> MAPAVAGGGRVRSNEPVAAAAAAPAASGKPCVCGFQVCACTGSAAVASAASSLDMDIVAMGQIGAVNDESWVGVELGEDGETDESGAAVDDRPVFRTEKIKGVLLHPYRVLIFVRLIAFTLFVIWRISHKNPDAMWLWVTSICGEFWFGFSWLLDQLPKLNPINRVPDLAVLRQRFDRPDGTSTLPGLDIFVTTADPIKEPILSTANSVLSILAADYPVDRNTCYVSDDSGMLLTYEALAESSKFATLWVPFCRKHGIEPRGPESYFELKSHPYMGRAQDEFVNDRRRVRKEYDEFKARINSLEHDIKQRNDGYNAAIAHSQGVPRPTWMADGTQWEGTWVDASENHRRGDHAGIVLVLLNHPSHRRQTGPPASADNPLDLSGVDVRLPMLVYVSREKRPGHDHQKKAGAMNALTRASALLSNSPFILNLDCDHYINNSQALRAGICFMVGRDSDTVAFVQFPQRFEGVDPTDLYANHNRIFFDGTLRALDGMQGPIYVGTGCLFRRITVYGFDPPRINVGGPCFPRLAGLFAKTKYEKPGLEMTTAKAKAAPVPAKGKHGFLPLPKKTYGKSDAFVDTIPRASHPSPYAAAAEGIVADEATIVEAVNVTAAAFEKKTGWGKEIGWVYDTVTEDVVTGYRMHIKGWRSRYCSIYPHAFIGTAPINLTERLFQVLRWSTGSLEIFFSKNNPLFGSTYLHPLQRVAYINITTYPFTAIFLIFYTTVPALSFVTGHFIVQRPTTMFYVYLGIVLSTLLVIAVLEVKWAGVTVFEWFRNGQFWMTASCSAYLAAVCQVLTKVIFRRDISFKLTSKLPSGDEKKDPYADLYVVRWTPLMITPIIIIFVNIIGSAVAFAKVLDGEWTHWLKVAGGVFFNFWVLFHLYPFA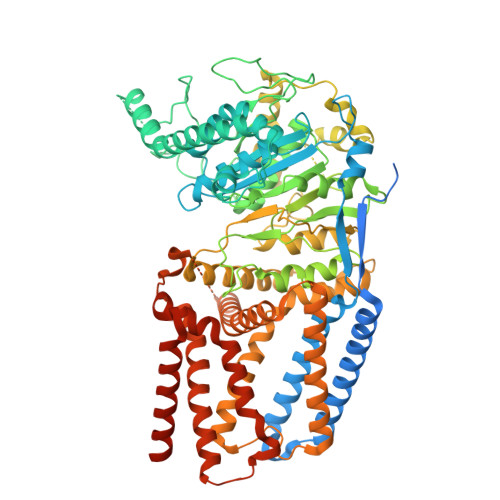KGILGKHGKTPVVVLVWWAFTFVITAVLYINIPHMHTSGGKHTTVHGHHGKKLVDTGLYGWLH>[3x]MGLGDPSVATVEDVSPTVFPAGPLFPTEGRIVQLFEKNTYSVVNIFDVTLRPQLKMTGVVEIPEGNGSGVVWDGQGYIVTNYHVIGNALSRNPSPGDVVGRVNILASDGVQKNFEGKLVGADRAKDLAVLKVDAPETLLKPIKVGQSNSLKVGQQCLAIGNPFGFDHTLTVGVISGLNRDIFSQTGVTIGGGIQTDAAINPGNAGGPLLDSKGNL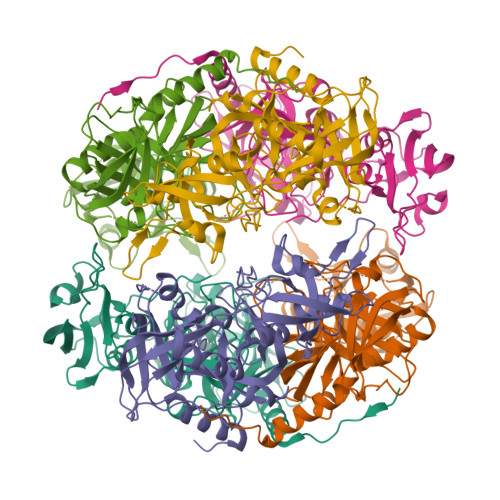IGINTAIFTQTGTSAGVGFAIPSSTVLKIVPQLIQFSKVLRAGINIELAPDPVANQLNVRNGALVLQVPGKSLAEKAGLHPTSRGFAGNIVLGDIIVAVDDKPVKNKAELMKILDEYSVGDKVTLKIKRGNEDLELKISLEEKSSLEHHHHHH> APQFFNIIDGSPLNFDDAMEEGRDTEAVKHFLETGENVYNEDPEILPEAEELYAGMCSGCHGHYAEGKIGPGLNDAYWTYPGNETDVGLFSTLYGGATGQMGPMWGSLTLDEMLRTMAWVRHLYTGDP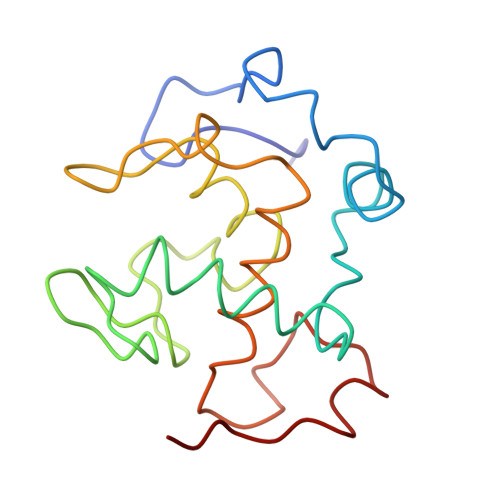KDASWLTDEQKAGFTPFQP>MLEYPIGTPQNLAGMEIAAVYLQPIDMEPEGHMRKASESDIHIEADIHALSNNPNGYPEGFWVPFLFIKYEITKVGGSGAPITGDMMAMVASDGPHYGDNVKLQGPGKYKVKYTIYPPNAKENPMSPYYGRHTDRETGVRPWFKTF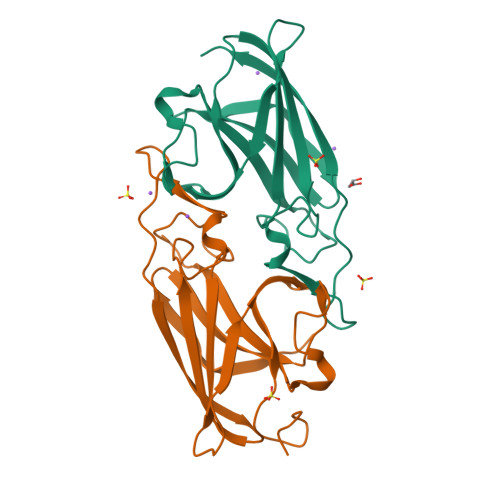SVEWDFTYAGIGKKGGY[2x]> MLRSLVQNPKVRARVLERVDEFRLNNLSNEEVWFRELTLCLLTANSSFISAYQALNCLGQKIYYANEEEIRNILKSCKYRFYNLKAKYIIMAREKV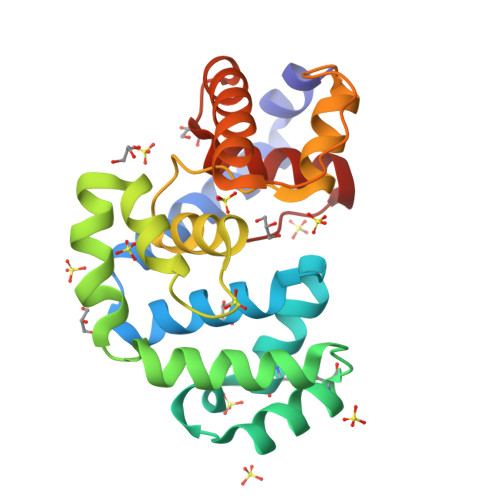YGRLKEEIKPLADEDQQLARERLLNIKGIGMQEASHFLRNVGYFDLAIIDRHIIDFMRRIGAIGETNVKQLSKSLYISFENILKSIASNLNMSVGILDLFIWYKETNTIVK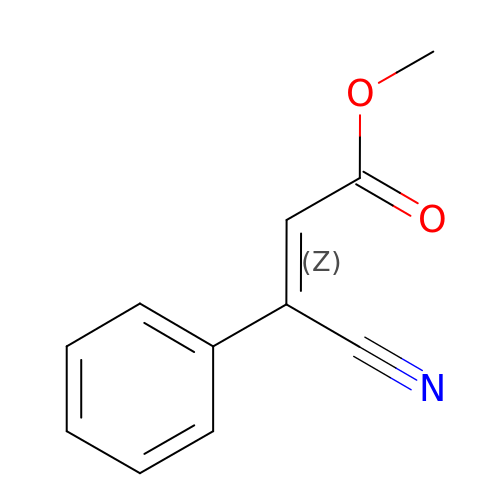methyl (2Z)-3-cyano-3-phenylprop-2-enoate | C11 H9 N O2 | GXUWXZSLWMEZET-JXMROGBWSA-N> MNARSTGQHPARYPGAAAGEPTLDSWQEPPHNRWAFAHLGEMVPSAAVSRRPVNAPGHALARLGAIAAQLPDLEQRLEQTYTDAFLVLRGTEVVAEYYRAGFAPDDRHLLMAVSKSLCGTVVGALVDEGRIDPAQPVTEYVPELAGSVYDGPSVLQVLDMQISIDYNEDYVDPASEVQTHDRSAGWGTRRHGDPADTYEFLTTLRGDGSTGEFQYCSANTD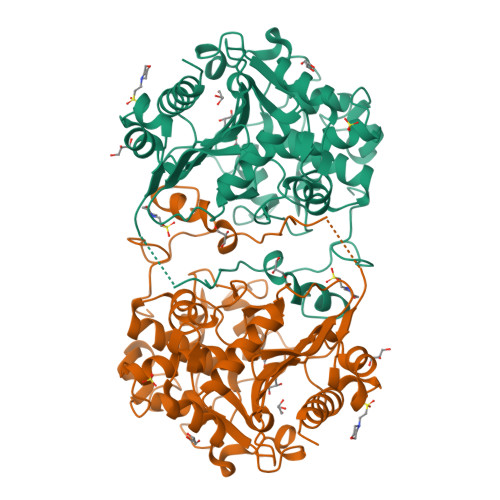VLAWIVERVTGLRYVEALSTYLWAKLDADRDATITVDTTGFGFANGGVSCTARDLARVGRMMLDGGVAPGGRVVSEDWVRRVLAGGSHEAMTDKGFTNTFPDGSYTRQWWCTGNERGNVSGIGIHGQNLWLDPLTDSVIVKLSSWPDPYTEHWHRLQNGILLDVSRALDAV>[2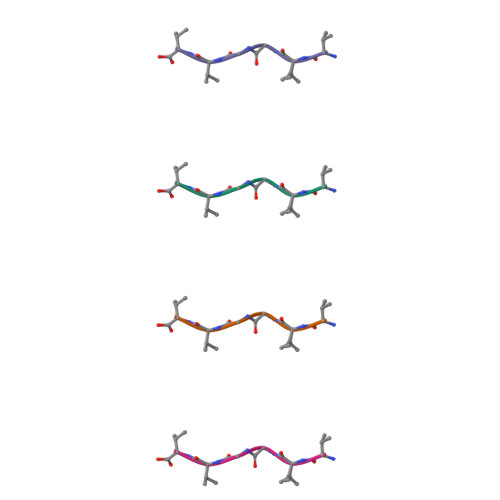x]VVGGVV>[2x]MGSSHHHHHHGSNQLTAYTLRLGDNCLVLSQRLGEWCGHAPELEIDLALANIGLDLLGQARNFLSYAAELAGEGDEDTLAFTRDERQFSNLLLVEQPNGNFADTI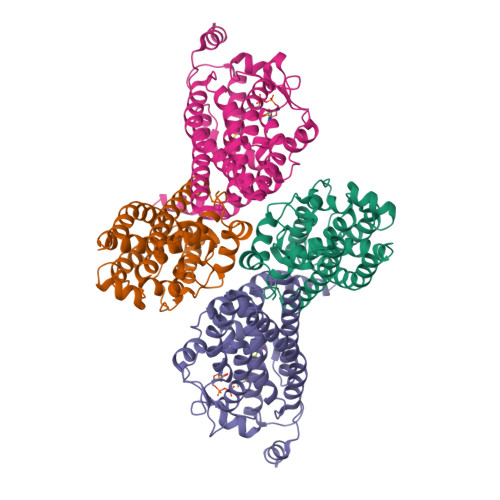ARQYFIDAWHVALFTRLMESRDPQLAAISAKAIKEARYHLRFSRGWLERLGNGTDVSGQKMQQAINKLWRFTAELFDADEIDIALSEEGIAVDPRTLRAAWEAEVFAGINEATLNVPQEQAYRTGGKKGLHTEHLGPMLAEMQYLQRVLPGQQW;>[2x]MRSTQEERFEQRIAQETAIEPQDWMPDAYRKTLIRQIGQHAHSEIVGMLPEGNWITRAPTLRRKAILLAKVQDEAGHGLYLYSAAETLGCAREDIYQKMLDGRMKYSSIFNYPTLSWADIGVIGWLVDGAAIVNQVALCRTSYGPYARAMVKICKEESFHQRQGFEACMALAQGSEAQKQMLQDAINRFWWPALMMFGPNDDNSPNSARSLTWKIKRFTNDELRQRFVDNTVPQVEMLGMTVPDPDLHFDTESGHYRFGEIDWQEFNEVINGRGICNQERLDAKRKAWEEGTWVREAALAHAQKQHARKVA> HKYKKQFRYESQLQMVQVTGSSDNEYFYVDFREYEYDLKWEFPRENLEFGKVLGSGAFGKVMNATAYGISKTGVSIQV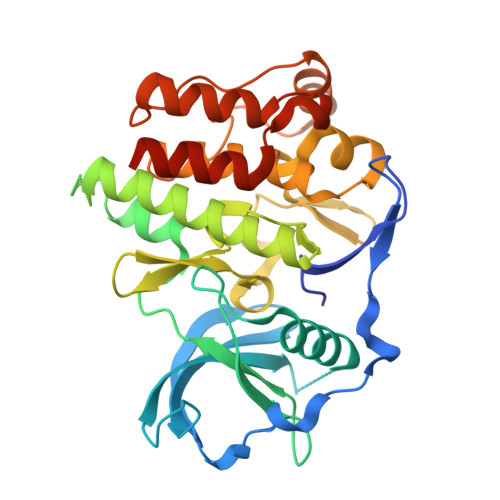AVKMLKEKADSSEREALMSELKMMTQLGSHENIVNLLGACTLSGPIYLIFEYCCYGDLLNYLRSKREKFSEDEIEYENQKRLEEEEDLNVLTFEDLLCFAYQVAKGMEFLEFKSCVHRDLAARNVLVTHGKVVKICDFGLARDIMSDSNYVVRGNARLPVKWMAPESLFEGIYTIKSDVWSYGILLWEIFSLGVNPYPGIPVDANFYKLIQNGFKMDQPFYATEEIYIIMQSCWAFDSRKRPSFPNLTSFLGCQLADAEEAMYQNV>[4x]SMGKLSEQLKHCNGILKELLSKKHAAYAWPFYKPVDAS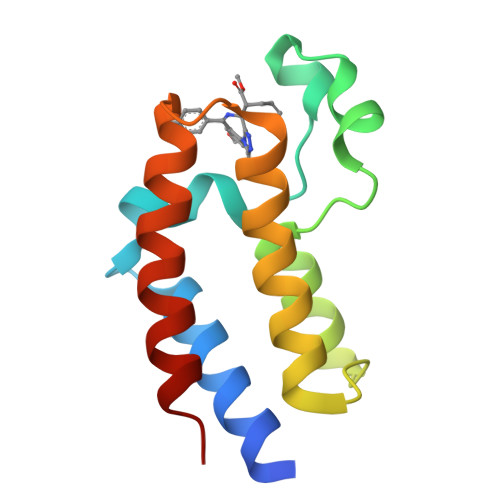ALGVHDYHDIIKHPMDLSTVKRKMENRDYRDAQEFAADVRLMFSNCYKYNPPDHDVVAMARKLQDVFEFRYAKMPD>[2x]MKYIIEHMEEGFSEWVILEYSQILREVGAENLILSSLPEST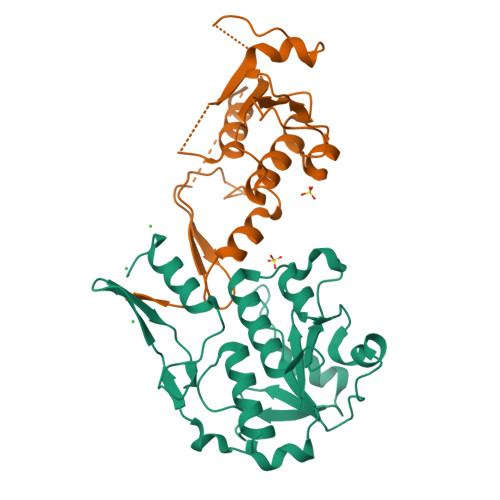TEKDIPQRLLKLGLRWTTKDLKGINEDFKDLELLKDGRVCLLDPRATIDLQPEDATKFDYFVFGGILGDHPPRDRTKELKTAYPNLLISRRLGDKQMTTDTAIRTTQLIIKDRIAFEDIKFIDYPEFRFNKNEATEMPFRYVLDKEGKPILPEGMLDLIKKDSLEHHHHHH>MPQDVDFHIPLPGRQSPDHARAEAEQLAWPRSLGLIR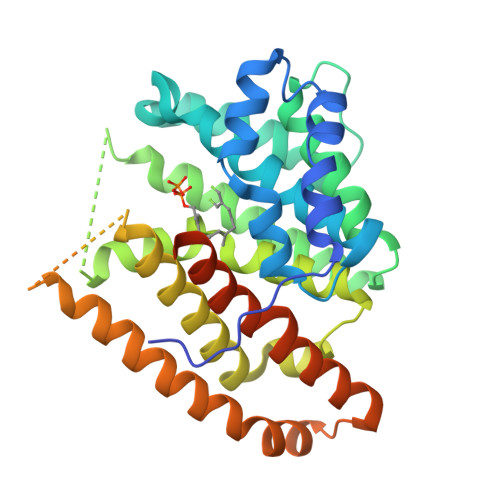SDAAAERHLRGGYADLASRFYPHATGADLDLGVDLMSWWFLFDDLFDGPRGENPEDTKQLTDQVAAALDGPLPDTAPPIAHGFADIWRRTCEGMTPAWCARSARHWRNYFDGYVDEAESRFWNAPCDSAAQYLAMRRHTIGVQPTVDLAERAGRFEVPHRVFDSAVMSAMLQIAVDVNLLLNDIASLEKEEARGEQNNMVMILRREHGWSKSRSVSHMQNEVRARLEQYLLLESCLPKVGEIYQLDTAEREALERYRTDAVRTVIRGSYDWHRSSGRYDAEFALAAGAQGYLEELGSSAH[2x]The serum glycoprotein leucine-rich ɑ-2-glycoprotein 1 (LRG1), primarily produced by hepatocytes and neutrophils, is a multifunctional protein that modulates various signaling cascades, mainly TGFβ signaling. Recently, we reported that the adhesion GPCR latrophilin-2 (LPHN2) is a TGF-β-independent receptor of LRG1, and the LRG1/LPHN2 axis exerts both angiogenic and neurotrophic effects under hyperglycemic conditions. LRG1, an LRR protein family member, comprises LRRNT, eight LRR repeats, and LRRCT.

The refined structure of LRG1 adopts a horseshoe-like solenoid structure that includes eight central LRR repeats (LRR1-LRR8) flanked by LRRNT and LRRCT domains. Similar to other typical LRR family members, each LRR repeat of LRG1 possesses a conserved LxxLxLxxNxL motif (where ‘x’ is any amino acid) composed of 24 amino acids. The concave face consists of parallel β-strands, whereas the convex surface comprises short 310 helices (R113-V115, V157-L160) or connecting loops. The LRRNT of LRG1 contains three β-strands, and its N-terminal β-hairpin is stabilized by only a single disulfide bridge that connects C43 and C56, whereas the LRRNT of other LRR families usually contains two disulfide bridges (top). The LRRCT of LRG1 contains one disulfide bond that connects C303 and C329 (bottom); thus, LRG1 belongs to the CF2 class. The electron density map of the LRG1 crystal structure and OMIT maps for glycans calculated by PHENIX42 clearly showed that N-acetylglucosamines are attached to four asparagine residues: N79 on LRRNT, N186 on the convex surface of LRR repeats, N269 on the concave surface of LRR repeats, and N325 on LRRCT. The glycans attached to N79, N269, and N325 were located on the same concave surface; among them, both N269 and N325 are highly conserved. However, O-linked glycosylation on T37 was not observed, because we could not build the three flexible residues (V36-L38) of LRG1. The structure prediction of the LRG1-cytochrome c complex using AlphaFold-multimer39 and the molecular docking of cytochrome c to LRG1 using Cluspro40 indicate that the conserved negatively charged residues in the concave surface of LRG1 (E76, E96, S100, D122, D194, E220, D266, S268, and D295) interact with the positively charged residues of cytochrome c (K9, K14, and K73). Specifically, the glycans on N325 of LRG1 LRRCT likely hinder LPHN2 binding, whereas the detachment of these glycans in a particular condition or a differential glycosylation mechanism relieves this steric hindrance, allowing the tight binding of LRG1 LRRCT to the LPHN2 Olf domain, similar to that in the FLRT2/LPHN3B complex.

> MSSWSRQRPKSPGGIQPHVSRTLFLLLLLAASAWGVTLSPKDCQVFRSDHGSSISCQPPAEIPGYLPADTVHLAVEFFNLTHLPANLLQGASKLQELHLSSNGLESLSPEFLRPVPQLRVLDLTRNALTGLPPGLFQASATLDTLVLKENQLEVLEVSWLHGLKALGHLDLSGNRLRKLPPGLLANFTLLRTLDLGENQLETLPPDLLRGPLQLERLHLEGNKLQVLGKDLLLPQPDLRYLFLNGNKLARVAAGAFQGLRQLDMLDLSNNSLASVPEGLWASLGQPNWDMRDGFDISGNPWICDQNLSDLYRWLQAQKDKMFSQNDTRCAGPEAVKGQTLLAVAKSQ>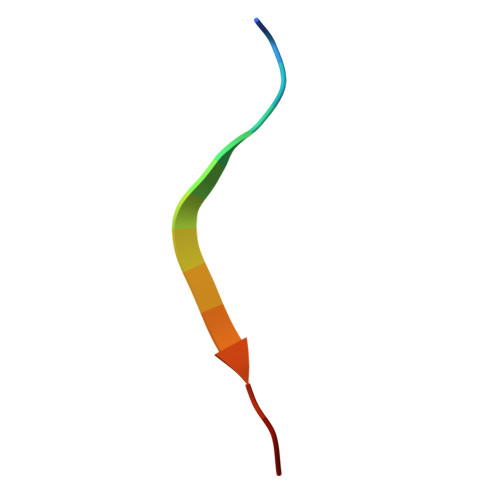 DSEPVLKGVKLHYT>[2x]GGDRVKKLINSQISLLIGKGLHEFDSLRDPEVNDFRTKMRQFCEEAAAHRQQLGWVEWLQYSFPLQLEPSARGWRAGLLRVSNRALLVNVKFEGSEESFTFQVSTKDMPLALMACALRKKATVFRQPLVEQPEEYALQVNGRHEYLYGNYPLCHFQYICSCLHSGLTPHLTMVHSSSILAMRDEQSNPAPQVQKPRAKPPPIPAKKPSSVSLWSLEQPFSIELIEGRKVNADERMKLVVQAGLFHGNEMLCKTVSSSEVNVCSEPVWKQRLEFDISVCDLPRMARLCFALYAVVEKAKKARSTKKKSKKADCPI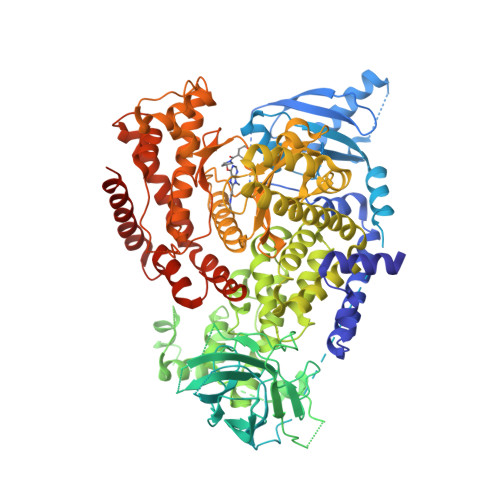AWANLMLFDYKDQLKTGERCLYMWPSVPDEKGELLNPAGTVRGNPNTESAAALVIYLPEVAPHPVYFPALEKILELGRHGERGRITEEEQLQLREILERRGSGELYEHEKDLVWKMRHEVQEHFPEALARLLLVTKWNKHEDVAQMLYLLCSWPELPVLSALELLDFSFPDCYVGSFAIKSLRKLTDDELFQYLLQLVQVLKYESYLDCELTKFLLGRALANRKIGHFLFWHLRSEMHVPSVALRFGLIMEAYCRGSTHHMKVLMKQGEALSKLKALNDFVKVSSQKTTKPQTKEMMHMCMRQETYMEALSHLQSPLDPSTLLEEVCVEQCTFMDSKMKPLWIMYSSEEAGSAGNVGIIFKNGDDLRQDMLTLQMIQLMDVLWKQEGLDLRMTPYGCLPTGDRTGLIEVVLHSDTIANIQLNKSNMAATAAFNKDALLNWLKSKNPGEALDRAIEEFTLSCAGYCVATYVLGIGDRHSDNIMIRESGQLFHIDFGHFLGNFKTKFGINRERVPFILTYDFVHVIQQGKTNNSEKFERFRGYCERAYTILRRHGLLFLHLFALMRAAGLPELSCSKDIQYLKDSLALGKTEEEALKHFRVKFNEALRESWKTKVNWLAHNVSKDNRQ> AGVVASQDQ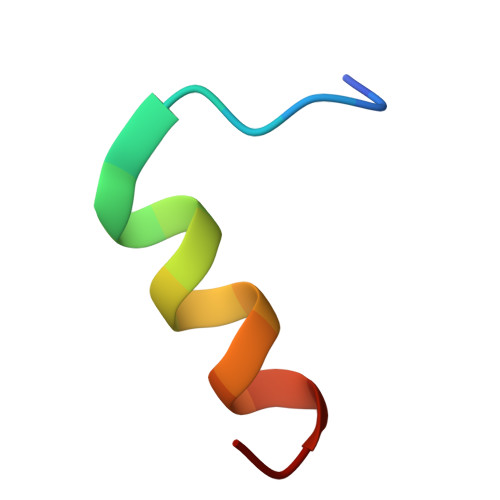VDDLLDSLGF> MGGVAMPGAEDDVVRENLYFQGKDGLAAMENAHTKTVEEVLGHFGVNESTGLSLEQVKKLKERWGSNELPAEEGKTLLELVIEQFEDLLVRILLLAACISFVLAWFEEGEETITAFVEPFVILLILVANAIVGVWQERNAENAIEALKEYEPEMGKVYRQDRKSVQRIKAKDIVPGDIVEIAVGDKVPADIRLTSIKSTTLRVDQSILTGESVSVIKHTDPVPDPRAVNQDKKNMLFSGTNIAAGKAMGVVVATGVNTEIGKIRDEMVATEQERTPLQQKLDEFGEQLSKVISLICIAVWIINIGHFNDPVHGGSWIRGAIYYFKIAVALAVAAIPEGLPAVITTCLALGTRRMAKKNAIVRSLPSVETLGCTSVICSDKTGTLTTNQMSVCRMFILDRVEGDTCSLNEFTITGSTYAPIGEVHKDDKPVNCHQYDGLVELATICALCNDSALDYNEAKGVYEKVGEATETALTCLVEKMNVFDTELKGLSKIERANACNSVIKQLMKKEFTLEFSRDRKSMSVYCTPNKPSRTSMSKMFVK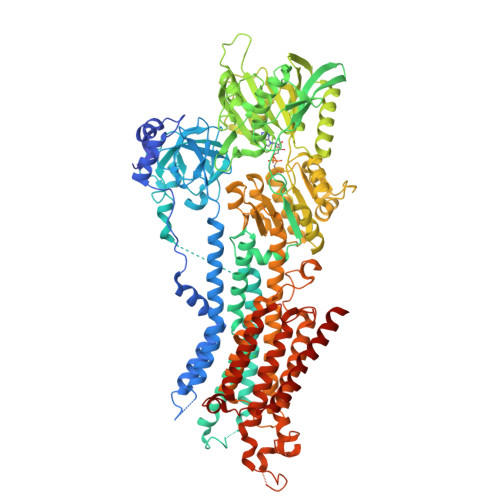GAPEGVIDRCTHIRVGSTKVPMTSGVKQKIMSVIREWGSGSDTLRCLALATHDNPLRREEMHLEDSANFIKYETNLTFVGCVGMLDPPRIEVASSVKLCRQAGIRVIMITGDNKGTAVAICRRIGIFGQDEDVTSKAFTGREFDELNPSAQRDACLNARCFARVEPSHKSKIVEFLQSFDEITAMTGDGVNDAPALKKAEIGIAMGSGTAVAKTASEMVLADDNFSTIVAAVEEGRAIYNNMKQFIRYLISSNVGEVVCIFLTAALGFPEALIPVQLLWVNLVTDGLPATALGFNPPDLDIMNKPPRNPKEPLISGWLFFRYLAIGCYVGAATVGAAAWWFIAADGGPRVSFYQLSHFLQCKEDNPDFEGVDCAIFESPYPMTMALSVLVTIEMCNALNSLSENQSLLRMPPWENIWLVGSICLSMSLHFLILYVEPLPLIFQITPLNVTQWLMVLKISLPVILMDETLKFVARNYLEPAILE> MGSDKIHHHHHHMAAFQIANKTVGKDAPVFIIAEAGINHDGKLDQAFALIDAAAEAGADAVKFQMFQADRMYQKDPGLYKTAAGKDVSIFSLVQSMEMPAEWILPLLDYCREKQVIFLSTVCDEGSADLLQSTSPSAFKIASYEINHLPLLKYVARLNRPMIFSTAGAEISDVHEAWRTIRAEGNNQIAIMHCVAKYPAPPEY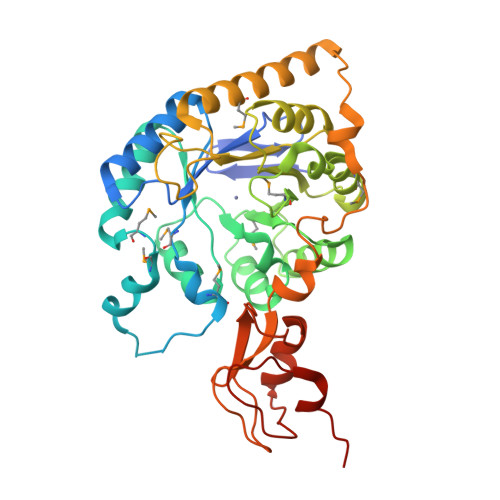SNLSVIPMLAAAFPEAVIGFSDHSEHPTEAPCAAVRLGAKLIEKHFTIDKNLPGADHSFALNPDELKEMVDGIRKTEAELKQGITKPVSEKLLGSSYKTTTAIEGEIRNFAYRGIFTTAPIQKGEAFSEDNIAVLRPGQKPQGLHPRFFELLTSGVRAVRDIPADTGIVWDDILLKDSPFHE>[4x]MDNEKKLFLKALKKKFEGEDPEEKSTNFYCFGGWEQSERKREFTEYAKKAAEKRGGIPFYNPDIGVPLGQRKLMAYRVSGTDAYVEGDDLHFVNNAAIQQMVDDIKRTVIVGMDTAHAVLEKRLGVEVTPETINEYMEVINHALPGGAVVQEHMVEVHPGIVEDCYAKVFTGDDNLADELDKRILIDINKEFPEEQAEQLKSYIGNRTYQVNRVPTIVVRACDGGTVSRWSAMQIGMSFISAYKLCAGEAAIADFSFAAKHADVIEMGTIMPARRARGPNEPGGVAFGTFADIVQASRVSDDPANVSLEVIAGAAALYDQVWLGSYMSGGVGFTQYATAAYTDDILDDFLYYGMEYVE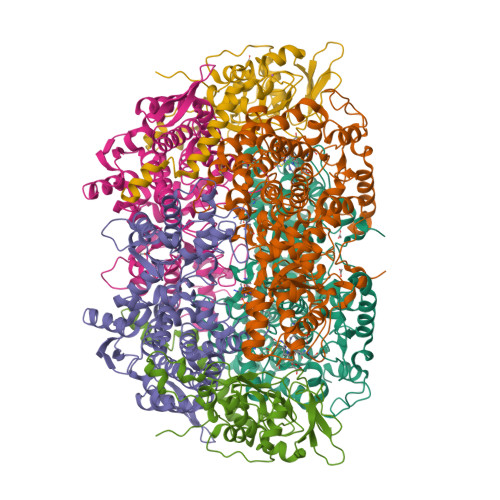DKFGICGSEPTMDVVRDISTEVTLYSLEQYEEYPTLLEDHFGGSQRAAVAAAAAGCSTAFATGNSNAGVNGWYLSQILHKEAHSRLGFYGYDLQDQCGASNSLSIRSDEGLIHELRGPNYPNYAMNVGHQPEYAGIAQAPHAARGDAFCTNPLIKVAFADKDLSFDFTSPRKSIAKGALREFIPEGERDLIIPAGK;>MPMYEDRVDLYGADGKLLEEDVPLEAVSPLKNPTIANLVSDVKRSVAVNLAGIEGSLRKAALGGKSNFIPGREVDLPIVENAEAIAEKIKKLVQTSEDDDTNIRLINNGQQILVQVPTTRMGVAADYTVSALVTGAAVVQAIIDEFDVDMFDANAVKTAVMGRYPQTVDFTGANLSTLLGPPVLLEGLGYGLRNIMANHVVAITRKNTLNASALSSILEQTAMFETGDAVGAFERMHLLGLAYQGLNANNLLFDLVKENGKGTVGTVIASLVERAIEDRVIKVAKEMTSGYKMYEPADWALWNAYAATGLLAATIVNVGAARAAQGVASTVLYYNDILEYETGLPGVDFGRAMGTAVGFSFFSHSIYGGGGPGIFHGNHVVTRHSKGFALPCVAAAMCLDAGTQMFSVEKTSGLIGSVYSEIDYFREPIVNVAKGAAEIKDQL[4x];>[4x]MSYKAQYTPGETRIAENRRKHMNPDYELRKLREISDEDLVKVLGHRNPGESYKSVHPPLDEMDFEEDIVRDLVEPIQGAKEGVRVRYIQFADSMYNAPAQPYDRARTYMWRYRGVDTGTLSGRQVIEMRELDLEGVSKELVETELFDPATTGIRGATVHGHSLRLDENGLMFDALQRYVFDEETGHVVYVKEQVGRPLDEPVDMGQPLDEEELRKITTIYRKDNIAMRDDKEAIEVVENIHTGRTMGGFGMDVFKEDLRKRLGDD>[2x]MGSDKIHHHHHHMETLILTQEE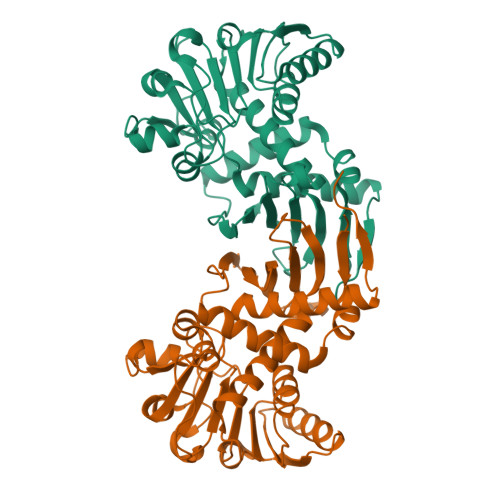VESLISMDEAMNAVEEAFRLYALGKAQMPPKVYLEFEKGDLRAMPAHLMGYAGLKWVNSHPGNPDKGLPTVMALMILNSPETGFPLAVMDATYTTSLRTGAAGGIAAKYLARKNSSVFGFIGCGTQAYFQLEALRRVFDIGEVKAYDVREKAAKKFVSYCEDRGISASVQPAEEASRCDVLVTTTPSRKPVVKAEWVEEGTHINAIGADGPGKQELDVEILKKAKIVVDDLEQAKHGGEINVAVSKGVIGVEDVHATIGEVIAGLKDGRESDEEITIFDSTGLAIQDVAVAKVVYENALSKNVGSKIKFFRI> XXXXXXXXXXXXXXXXXXXXXXXXXXXXXXXXXXXXXXXXXXXXXXXXXXXXXXXXXXXXXXXXXXXKLTLGLSILFMVEAAEFTVPKKDLDSLCYLLIPSAGSPEALHSDLSPVLRIRQRWRIYLTNLCLRCIDERCDRWLGILPLLHTCMQKSPPKKNSKSQPEDTWAGLEGISFSEFRDKAPTRSQPLQFMQSKMALLRVDEYLFRSWLSVVPLESLSSYLENSIDYLSDVPVRVLDCLQGISYRLPGLRKISNQNMKKDVENVFKMLMHLVDIYQHRIFGENLLQIYLTECLTLHETVCNITANHQFFEIPALSAELICKLLELSPPGHTDEGLPEKSYEDLVTSTLQEALATTRNWLRSLFKSRMLSISSAYVRLTYSEEMAVWRRLVEIGFPEKHGWKGSLLGDMEGRLKQEPPRLQISFFCSSQCRDGGLHDSVSRSFEKCVIEAVSSACQSQTSVLEGLSCQDLQKFGTLLSAVITKSWPVHNGEPVFDVDEIFKYLLKWPDVRQLFELCGTNEKIIDNITEEGRQLMATAESVFQKVAGELENGTIVVGQLELILEHQSQFLDIWNLNRRRLPSQEKACDVRSLLKRRRDDLLFLKQEKRYVESLLRQLGRVKHLVQVDFGNIEIIHSQDLSNKKLNEAVIKLPNSSSYKRETHYCLSPDIREMASKLDSLKDSHIFQDFWQETAESLNTLDKDPRELKVSLPEVLEYLYNPCYDNFYTLYENLKSGKITFAEVDAIFKDFVDKYDELKNDLKFMCTMNPQDQKGWISERVGQIKEYHTLHQAVSSAKVILQVRRALGVTGDFSVLNPLLNFADSFEDFGNEKLDQISPQFIKAKQLLQDISEPRQRCLEELARQTELVAWLHKALEDINELKVFVDLASISAGENDIDVDRVACFHDAVQGYASLLYKMDERTNFSDFMNHLQELWRALDNDQHLPDKLKDSARNLEWLKTVKESHGSVELSSLSLATAINSRGVYVIEAPKDGQKISPDTVLRLLLPDGHGYPEALRTYSTEELKELLNKLMLMSGKKDHNSNTEVEKFSEVFSNMQRLVHVFIKLHCAGNMLFRTWTAKVYCCPDGGIFMNFGLELLSQLTEKGDVIQLLGALCRQMEDFLDNWKTVVAQKRAEHFYLNFYTAEQLVYLSSELRKPRPSEAALMMLSFIKGKCTVQDLVQATSACESKADRYCLREVMKKLPQQLLSEPSLMGKLQVIMMQSLVYMSAFLPHCLDLDALGRCLAHLATMGGTPVERPLPKGLQAGQPNLILCGHSEVLPAALAIYMQAPRQPLPTFDEVLLCTPATTIEEVELLLRRCLTSGSQGHKVYSLLFADQLSYEVGCQAEEFFQSLCTRAHREDYQLVILCDAAREHCYIPSTFSQYKVPLVPQAPLPNIQAYLQSHYQVPKRLLSAATVFRDGLCVGIVTSERAGVGKSLYVNTLHTKLKAKLRDETVPLKIIRLTEPHLDENQVLSALLPFLKEKYQKMPVIFHIDISTSVQTGIPIFLFKLLILQYLMDINGKIWRRSPGHLYLVEIPQGLSVQPKRSSKLNARAPLFKFLDLFPKVTCRPPKEVIDMELTPERSHTDPAMDPVEFCSEAFQRPYQYLKRFHQQQNLDTFQYEKGSVEGSPEECLQHFLIYCGLINPSWSELRNFAWFLNCQLKDCEASIFCKSAFTGDTLRGFKNFVVTFMILMARDFATPTLHTSDQSPGRQSVTIGEVVEEDLAPFSLRKRWESEPHPYVFFNGDHMTMTFIGFHLETNNNGYVDAINPSNGKVIKKDVMTKELFDGLRLQRVPFNIDFDNLPRYEKLERLCLALGIEWPIDPDETYELTTDNMLKILAIEMRFRCGIPVIIMGETGCGKTRLIKFLSDLKRGSVEAETMKLVKVHGGTTPSMIYSKVKEAERTAFSNKAQHKLDTILFFDEANTTEAVSCIKEILCDRTVDGEHLHEDSGLHIIAACNPYRKHSQEMILRLESAGLGYRVSAEETADRLGSIPLRQLVYRVHALPPSLIPLVWDFGQLNDSAEKLYIQQIVQRLVDSVSVNPSETCVIADVLSASQMFMRKRENECGFVSLRDVERCVKVFRWFHDHSDMLLKELDKFLHESSDSTHTFERDPVLWSLVMAIGVCYHASLEEKASYRTAIARCFPKPYNSSRAILDEVTHVQDLFLRGAPIRTNIARNLALKENVFMMVICIELKIPLFLVGKPGSSKSLAKIIVADAMQGQAAFSELFRCLKQVHLVSFQCSPHSTPQGIISTFKQCARFQQGKDLGQYVSVVVLDEVGLAEDSPKMPLKTLHPLLEDGCIEDDPAPYKKVGFVGISNWALDPAKMNRGIFVSRGSPNEKELIESAEGICSSDRLVQDKIRGYFAPFAKAYETVCQKQDKEFFGLRDYYSLIKMVFAKAKASKRGLSPQDITHAVLRNFSGKDNIQALSIFTASLPEARYKEEVSTVELIKQNIYPGPQASSRGLDGAESRYLLVLTRNYVALQILQQTFFEGQQPEIIFGSSFPQDQEYTQICRNINRVKICMETGKMVVLLNLQNLYESLYDALNQYYVYLGGQKYVDLGLGTHRVKCRVHTAFRLIVIEEKDVVYKQFPVPLINRLEKHYLDMNTVLQPWQKSIVQELQQWAHEFADVKADQFIARHKYSPADVFIGYHSDACASVVLQAVERQGCRDLTEELYRKVSEEARSILLDCATPDAVVRLSGSSLGSFTAKQLSQEYYYAQQHNSFVDFLQAHLRMTHHECRAVFTEITTFSRLLTGNDCDVLASELRGLASKPVVLSLQQYDTEYSFLKDVRSWLTNPGKRKVLVIQADFDDGTRSAQLVASAKYTAINEINKTQGTKDFVFVYFVTKLSRMGSGTSYVGFHGGLWRSVHIDDLRRSTIMASDVTKLQNVTISQLFKPEDKPEQEEMEIETSQSKELAEEQMEVEDSEEMKKASDPRSCDCSQFLDTTRLVQSCVQGAVGMLRDQNESCARNMRRVTILLDLLNEDNTRNASFLRESKMRLHVLLNKQEENQVRSLKEWVTREAANQDALQEAGTFRHTLWKRVQDVVTPILASMIAHIDRDGNLELLAQPDSPAWVQDLWMFIYSDIKFLNISLVLNNTRSNSEMSFILVQSHMNLLKDAYNAVPFSWRIRDYLEELWVQAQYITDTEGLSKKFVEIFQKTPLGVFLAQFPVAQQQKLLQSYLKDFLLLTMKVSSREELMFLQMALWSCLRELQEASGTPDETYKFPLSLPWVHLAFQHFRTRLQNFSRILTIHPQVLSSLSQAAEKHSLAGCEMTLDAFAAMACAEMLKGDLLKPSPKAWLQLVKNLSTPLELVCSEGYLCDSGSMTRSVIQEVRALWNRIFSIALFVEHVLLGTESHIPELSPLVTTYVS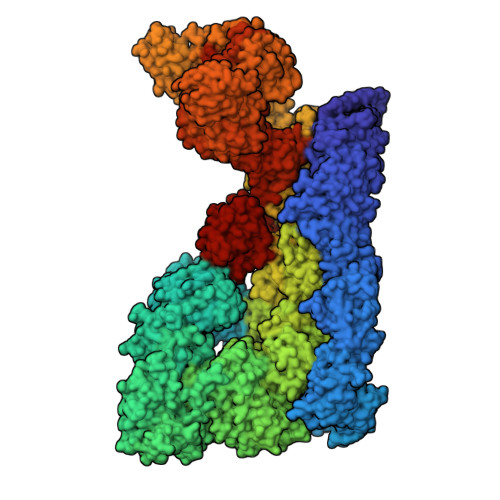LLDKCLEEDSNLKTCRPFVAVMTTLCDCKDKASKKFSRFGIQPCFICHGDAQDPVCLPCDHVYCLRCIQTWLIPGQMMCPYCLTDLPDKFSPTVSQDHRKAIEKHAQFRHMCNSFFVDLVSTMCFKDNTPPEKSVIDTLLSLLFVQKELLRDASQKHREHTKSLSPFDDVVDQTPVIRSVLLKLLLKYSFHEVKDYIQNYLTQLEKKAFLTEDKTELYLLFISCLEDSVHQKTSAGCRNLEQVLREEGHFLRTYSPGLQGQEPVRIASVEYLQEVARVRLCLDLAADFLSELQEGSELAEDKRRFLKHVEEFCTRVNNDWHRVYLVRKLSSQRGMEFVQSFSKQGHPCQWVFPRKVIAQQKDHVSLMDRYLVHGNEYKAVRDATAKAVLECKTLDIGNALMACRSPKPQQTAYLLLALYTEVAALYRSPNGSLHPEAKQLEAVNKFIKESKILSDPNIRCFARSLVDNTLPLLKIRSANSILKGTVTEMAVHVATILLCGHNQILKPLRNLAFYPVNMANAFLPTMPEDLLVHARTWRGLENVTWYTCPRGHPCSVGECGRPMQESTCLDCGLPVGGLNHTPHEGFSAIRNNEDRTQTGHVLGSPQSSGVAEVSDRGQSPVVFILTRLLTHLAMLVGATHNPQALTVIIKPWVQDPQGFLQQHIQRDLEQLTKMLGRSADETIHVVHLILSSLLRVQSHGVLNFNAELSTKGCRNNWEKHFETLLLRELKHLDKNLPAINALISQDERISSNPVTKIIYGDPATFLPHLPQKSIIHCSKIWSCRRKITVEYLQHIVEQKNGKETVPVLWHFLQKEAELRLVKFLPEILALQRDLVKQFQNVSRVEYSSIKGFIHSHSSDGLRKLLHDRITIFLSTWNALRRSLETNGEIKLPKDYCCSDLDLDAEFEVILPRRQGLGLCGTALVSYLISLHNNMVYTVQKFSNEDNSYSVDISEVADLHVISYEVERDLNPLILSNCQYQVQQGGETSQEFDLEKIQRQISSRFLQGKPRLTLKGIPTLVYRRDWNYEHLFMDIKNKMAQSSLPNLAISTISGQLQSYSDACEALSIIEITLGFLSTAGGDPGMDLNVYIEEVLRMCDQTAQVLKAFSRCQLRHIIALWQFLSAHKSEQRLRLNKELFREIDVQYKEELSTQHQRLLGTFLNEAGLDAFLLELHEMIVLKLKGPRAANSFNPNWSLKDTLVSYMETKDSDILSEVESQFPEEILMSSCISVWKIAATRKWDRQSRGGGHHHHHHHHHH> AQSVPYGVSQIKAPALHSQGYTGSNVKVAVIDSGIDSSHPDLNVAGGASFVPSETNPFQDNNSHGTHVAGTVLAVAPSASLYAVKVLGADGSGQYSWIINGIEWAIANNMDVINMSLGGPSGSAALKAAVDKAVASGVVVVAAAGNEGTSGSSSTVGYPGKYPSVIAVGAVDSSNQRASFSSVGPELDVMAPGVSIVSTLPGNKYGAKSGTAMASPHVAGAAALILSKHPNWTNTQVRSSLENTTTKLGDSFYYGKGL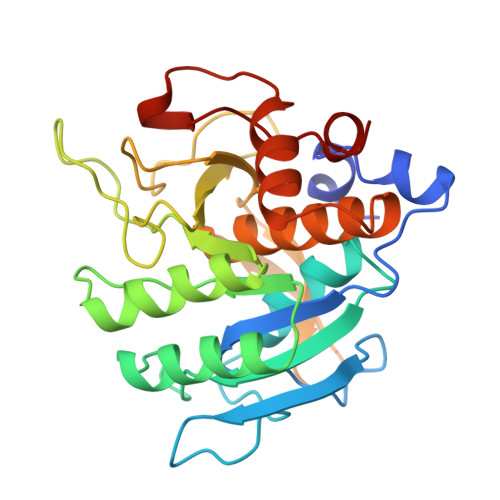INVEAAAQ> MTNIDVRWQQRLNNYARALQQLSLAVNLAQTRPLSDLEKQGLIQAFEFTHELAWNVMKDYFFFQGNSAITGSRDATRESFNKGLIKEGEIWMEMIKSRNQTSHTYNQ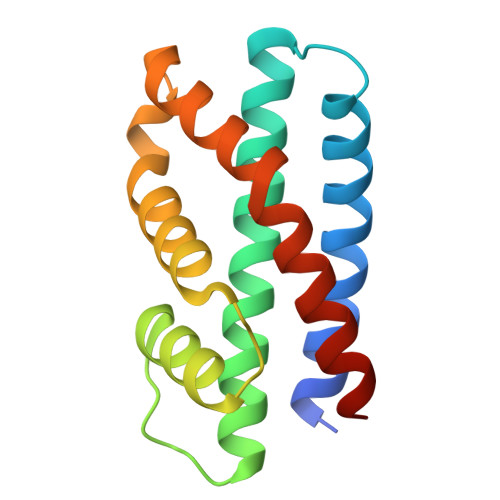SVADEIVKNIINFYHTSFQAFLEKMQGLKEHE> MATRGHVQDPNDRRLRPIYDYLDNGNNKMAIQQADKLLKKHKDLHCAKVLKAIGLQRTGKQEEAFTLAQEVAALEPTDDNSLQALTILYREMHRPELVTKLYEAAVKKVPNSEEYHSHLFMAYARVGEYKKMQQAGMALYKIVPKNPYYFWSVMSLIMQSISAQDENLSKTMFLPLAERMVEKMVKEDKIEAEAEVELYYMILERLGKYQEALDVIRGKLGEKLTSEIQSRENKCMAMYKKLSRWPECNALSRRLLLKNSDDWQFYLTY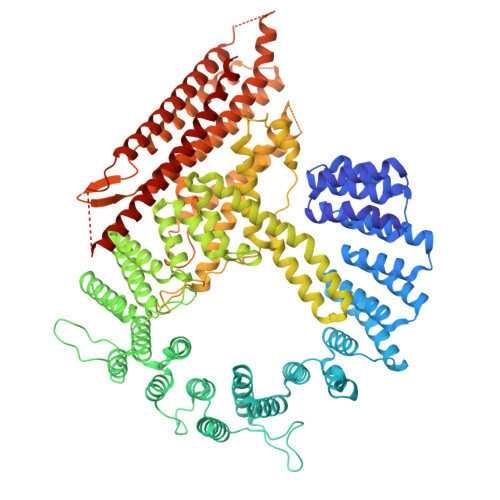FDSVFRLIEEAWSPPAEGEHSLEGEVHYSAEKAVKFIEDRITEESKSSRHLRGPHLAKLELIRRLRSQGCNDEYKLGDPEELMFQYFKKFGDKPCCFTDLKVFVDLLPATQCTKFINQLLGVVPLSTPTEDKLALPADIRALQQHLCVVQLTRLLGLYHTMDKNQKLSVVRELMLRYQHGLEFGKTCLKTELQFSDYYCLLAVHALIDVWRETGDETTVWQALTLLEEGLTHSPSNAQFKLLLVRIYCMLGAFEPVVDLYSSLDAKHIQHDTIGYLLTRYAESLGQYAAASQSCNFALRFFHSNQKDTSEYIIQAYKYGAFEKIPEFIAFRNRLNNSLHFAQVRTERMLLDLLLEANISTSLAESIKSMNLRPEEDDIPWEDLRDNRDLNVFFSWDPKDRDVSEEHKKLSLEEETLWLRIRSLTLRLISGLPSLNHPVEPKNSEKTAENGVSSRIDILRLLLQQLEATLETGKRFIEKDIQYPFLGPVPTRMGGFFNSGCSQCQISSFYLVNDIYELDTSGLEDTMEIQERIENSFKSLLDQLKDVFSKCKGDLLEVKDGNLKTHPTLLENLVFFVETISVILWVSSYCESVLRPYKLNLQKKKKKKKETSIIMPPVFTSFQDYVTGLQTLISNVVDHIKGLETHLIALKLEELILEDTSLSPEERKFSKTVQGKVQSSYLHSLLEMGELLKKRLETTKKLKI2-[5-[(1~{R},2~{R},4~{S})-7-azabicyclo[2.2.1]heptan-2-yl]-2-fluoranyl-pyridin-3-yl]pyridine-4-carboxamide | C17 H17 F N4 O | 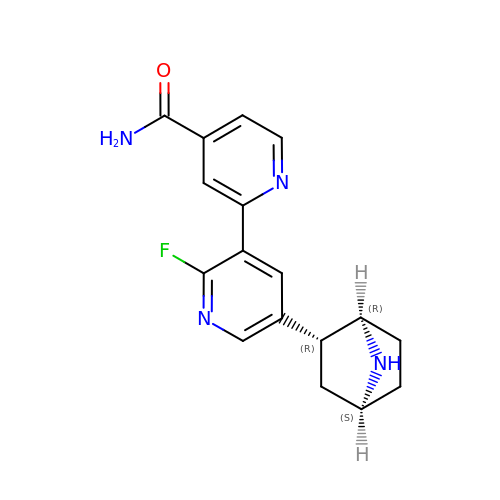FQBYLVVJPBRDCG-OUCADQQQSA-N> MEYQRAIDSIEECLNKQLRLSSEK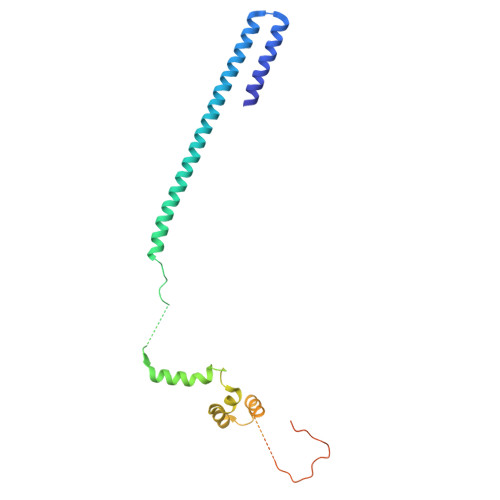VDQYVLIENWTSLVGHLKTLHSLISNYTNGRELQNEISSLLKQDKELDLQIQDCMREMTSIYDTHLPKTVSGRKRQKVNAETLLDYGRKLSKFSSAPPGYNPETGQDAKAPVHYPWPSEDQMRKTLLFQFSTSMVPNLSATASQLFSEQPPKTNEPTETETEIDANKAVEEKTKMNYPASPTFTTQEENKEVESPANKDVFAGFDLFDPEMEEDF>MITVFGL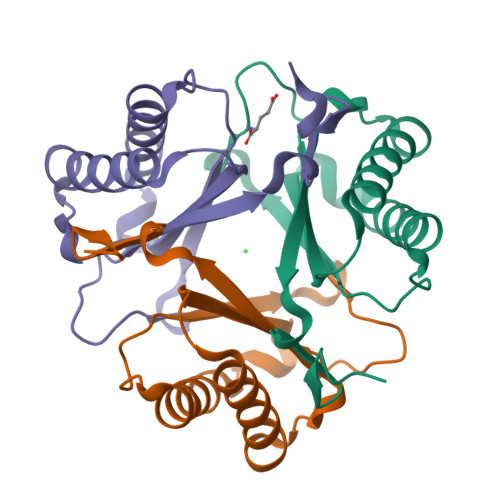KSKLAPRREKLAEVIYNSLHLGLDIPKGKHAIRFLCLEKEDFYYPFDRSDDYTVIEINLMAGRMEGTKKRLIKMLFSELEYKLGIRAHDVEITIKEQPAHCWGFRGMTGDEARDLDYDIYV[3x]>[6x]MD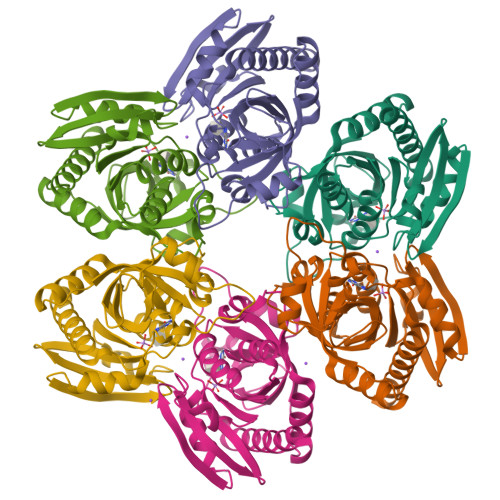NLLRHLKISKEQITPVVLVVGDPGRVDKIKVVCDSYVDLAYNREYKSVECHYKGQKFLCVSHGVGSAGCAVCFEELCQNGAKVIIRAGSCGSLQPDLIKRGDICICNAAVREDRVSHLLIHGDFPAVGDFDVYDTLNKCAQELNVPVFNGISVSSDMYYPNKIIPSRLEDYSKANAAVVEMELATLMVIGTLRKVKTGGILIVDGCPFKWDEGDFDNNLVPHQLENMIKIALGACAKLATKYALEHHHHHH>MTLGTNQVSKTHSFMTVSLIELWERFGYYGMQALIVYFMVQRLGFDDSRANLVWSACAALIYVSPAIGGWVGDKILGTKRTMLLGAGILSVGYALMTVPTENTWFMFSALGVIVVGNGLFKPNAGNLVRKIYEGDDSKIDSAFTIYYMAVNVGSTFSMLLTPWIKDYVNAQYGNEFGWHAAFAVCCVGILVGLGNYALMHKSLANYGSEPDTRPVNKKSLAIVLALAALSVVASAIILEYEDVARVFVYAAGVAVLGIFFHLIRTSEPSERAGLIAALILTVQTVFFF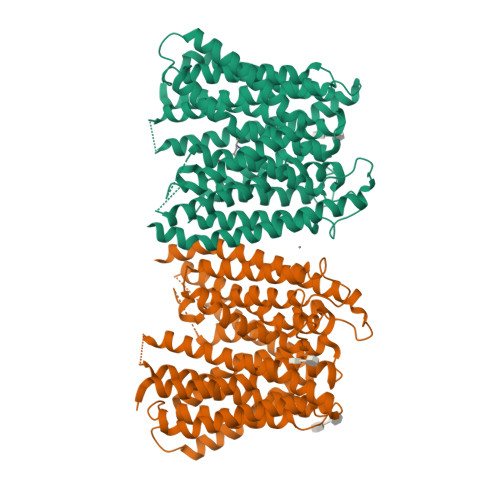IFYQQMSTSLALFALRNVDWDFQVFGTHLWTWSPAQFQALNPIWIMVLSPVLAWSYSWAGRNNKDFSIAAKFALGFAVVAIGFFIYGFAGQFAVNGKTSSWVMIWGYASYSLGELLVSGLGLAMIARYVPARMGGFMMGAYFVASGISQYLGGVVANFASVPQDLVDPLQTLPVYTNLFNKLGVAAVVCTIIALAVLPLMRRLTESHHAHSSIENNAAASLRDVKAEQAENLYFQ[2x]6-O-methyl-beta-D-galactopyranose 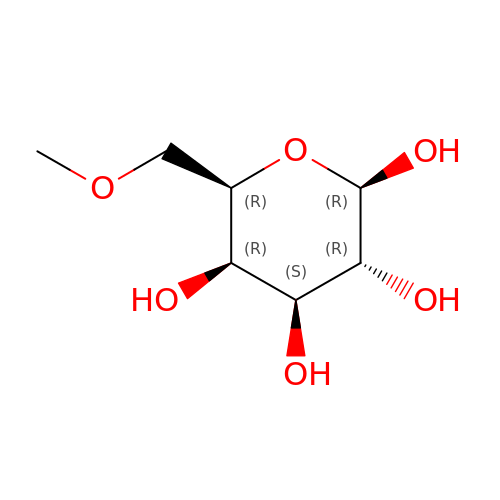| C7 H14 O6 | QWJKEQVWXSYDJA-VOQCIKJUSA-N>[4x]GSLHMSFETRFEKMDNLLRDPKSEVNSDCLLDGLDALVYDLDFPALRKNKNIDNFLSR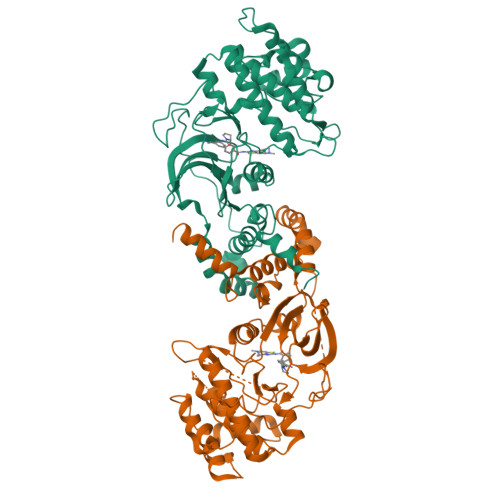YKDTINKIRDLRMKAEDYEVVKVIGRGAFGEVQLVRHKSTRKVYAMKLLSKFEMIKRSDSAFFWEERDIMAFANSPWVVQLFYAFQDDRYLYMVMEYMPGGDLVNLMSNYDVPEKWARFYTAEVVLALDAIHSMGFIHRDVKPDNMLLDKSGHLKLADFGTCMKMNKEGMVRCDTAVGTPDYISPEVLKSQGGDGYYGRECDWWSVGVFLYEMLVGDTPFYADSLVGTYSKIMNHKNSLTFPDDNDISKEAKNLICAFLTDREVRLGRNGVEEIKRHLFFKNDQWAWETLRDTVAPVVPDLSSDIDTSNFDDLEEDKGEEETFPIPKAFVGNQLPFVGFTYYSNRRYLSSANPNDNR>[2x]MTRDQNGTWEMESNENFEGYMKALDIDFATRKIAVRLTQTKVIDQDGDNFKTKTTSTFRNYDVDFTVGVEFDEYTKSLDNRHVKALVTWEGDVLVCVQKGEKENRGWKQWIEGDKLYLELTCGDQVCRQVFKKKLVPR

Present in the small intestine, cellular retinol binding protein 2 (CRBP2) plays an important role in the uptake, transport, and metabolism of dietary retinoids. All CRBPs share the same protein structure architecture. These small soluble proteins fold into a single β-barrel that shields the central hydrophobic cavity that constitutes a solitary binding site for retinoids. Access to the binding pocket is governed by a “portal region” composed of conformationally flexible loops connecting neighboring β-strands. By examining chemical libraries of bioactive lipids, we provided evidence for the selective interaction of CRBP2 with a subset of nonretinoid ligands with the highest affinity for sn-1 and sn-2 MAGs that contain polyunsaturated C18-C20 acyl chains.

1-arachidonoylglycerol (1-AG) interacts with CRBP2 with a Kd of 37.9 ± 3.3 nM. In fact, as discussed later in this report, only 1-AG (S-isomer) binds to CRBP2. Indeed, the crystal structure of CRBP2 in the complex with 1-AG clearly indicates that despite geometrical differences between 2-AG and its sn-1 and sn-3 isomers, the binding modes for both molecules are identical. Inside the binding cavity, the arachidonoyl chains of 1-AG and 2-AG adapted the same orientations enforced by hydrophobic and van Der Waals interactions with the side chains of the enclosed portal region of the protein. Also, the position of the oxygen atoms of the ester bonds were nearly overlapping (root-mean-square deviation of atomic positions, 0.3 Å), as they were locked in place by hydrogen bonds between the carboxyl oxygen and an ordered water molecule (W1) as well as the potential interaction of the ester oxygen with the ζ amino group of K40. Similarly, the nonesterified hydroxyl groups of both ligands were engaged in the same network of hydrogen bonds that involved the side chains of K40, T51, and Q108. Thus, the identical contact points between these ligands and the protein observed for 1-AG and 2-AG could be achieved only by adapting an alternative orientation of the glycerol backbones in the binding pocket (root-mean-square deviation value for the glycerol carbon atoms = 1.3 Å). The only consequence of this difference is the 1 Å shift of the sn-3 hydroxyl group toward the location normally occupied by an ordered water (W2) in the 2-AG/CRBP2 complex. Thus, this water molecule is no longer present in the structure of 1-AG. Importantly, the binding of MAGs by CRBP2 is restricted to sn-1 and sn-2 isomers. Despite the use of a racemic mixture of 1-AG and 3-AG in the crystallographic experiments, the electron density for the ligand clearly indicated the exclusive presence of 1-AG (S-enantiomer) in the binding pocket.6-BENZYL-5-CHLORO-7-HYDROXYPYRAZOLO[1,5-A]PYRIMIDINE-3-CARBOXYLIC 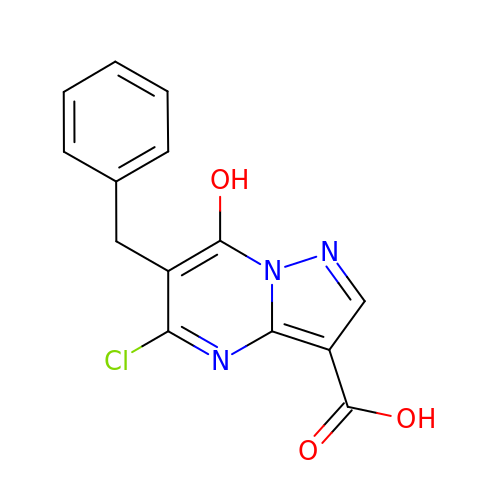ACID | C14 H10 Cl N3 O3 | AMDMCXLZDLJCSY-UHFFFAOYSA-N> MSKLLMIGTGPVAIQLANICYLKSDYEIDMVGRASTSEKSKRLYQAYKKEKQFEVKIQNEAHQHLEGKFEINRLYKDVKNVKGEYETVVMACTADAYYDTLQQLSLETLQSVKHVILISPTFGSQMIVEQFMSKFSQDIEVISFSTYLGDTRIVDKEAPNHVLTTGVKKKLYMGSTHSNSTMCQRISALAEQLKIQLEVVESPLHAETRNSSLYVHPPLFMNDFSLKAIFEGTDVPVYVYKLFPEGPITMTLIREMRLMWKEMMAILQAFRVPSVNLLQFMVKENYPVRPETLDEGDIEHFEILPDILQEYLLYVRYTAILIDPFSQPDENGHYFDFSAVPFKQVYKNEQDVVQIPRMPSEDYYRTAMIQHIGKMLGIKTPMIDQFLTRYEASCQAYKDMHQDQQLSSQFNTNLFEGDKALVTKFLEINRTLSKGELNSKLEGKPIPNPLLGLDSTR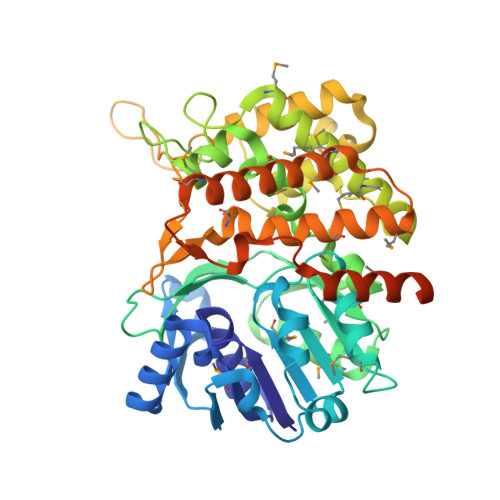TGHHHHHH>[9x]MDWHIAKHYDDILYYKAGGIAKIVINRPHKRNAFRPQTVFELYDAFCNAREDNRIGVVLLTGAGPHSDGKYAFCSGGDQSVRGEGGYIDDQGTPRLNVLDLQRLIRSMPKVVIALVAGYAIGGGHVLHLVCDLTIAADNAIFGQTGPKVGSFDGGFGSSYLARIVGQKKAREIWYLCRQYSAQEAERMGMVNTVVPVDRLEEEGIQWAKEILSKSPLAIRCLKAAFNADCDGQAGLQELAGNATLLYYMTEEGSEGKQAFLEKRPPDFSQYPWLP

1, 4-Dihydroxy-2-naphthoyl-CoA (DHNA-CoA) synthase, also called MenB, is responsible for conversion of o-succinylbenzoyl-CoA to DHNA-CoA in the biosynthesis of both vitamin K1 and K2. It catalyzes a multiple-step intramolecular Claisen condensation reaction involving two high energy oxyanion intermediates and two keto-enol tautomerizations in the formation of a naphthenoid ring. The first crystal structure of DHNA-CoA synthase from Mycobacterium tuberculosis shows that it forms two eclipsed trimers organized in a homologous hexameric assembly, in which each monomer is comprised of an N-terminal spiral core domain and a C-terminal helical domain conforming to a canonical crotonase fold. In addition to observing the folding of the active-site loop into a well-defined structure as previously seen in the substrate analog complex structure, we have identified a significant reorientation of the C-terminal helix as an additional conformational change caused by the small molecule ligands.

Through symmetry operation, all the trimers are found to be a part of the hexameric quaternary structure of scMenB. The active site of scMenB in complex with SA-CoA is also very similar to that of the ecMenB:HNA-CoA and scMenB:HNA-CoA complexes. However, no hydrogen-bonding network is found in the scMenB:SA-CoA structure. In addition, a bicarbonate ion is found in the place of the chloride ion in the ecMenB:HNA-CoA or scMenB:HNA-CoA structure. scMenB forms identical polar and nonpolar contacts with the adenylate moiety of HNA-CoA and SA-CoA in the complexes, but shows differences when compared to ecMenB. One of them is a strong hydrogen bond between the strictly conserved A-loop Arg-82 and the backbone carbonyl oxygen of the C-helix Gly-253, and the other polar loop-helix interaction is a hydrogen bond between the backbone carbonyl oxygen of Arg-82 and the side chain guanidinium group of Lys-257. For example, the side chain of scMenB Leu-261 on the C-helix forms hydrophobic contact with the A-loop, which replaces the interfacial hydrogen bond formed by the corresponding amino acid residue Asn-271 on the ecMenB C-helix. In addition, the adenylate 3′-phosphate group of the ligand is also stabilized by a ligand-induced salt bridge with the side chain of scMenB Lys-263, which is equivalent to ecMenB Lys-273. In the scMenB complexes, the lp−π interaction is formed between the purine moiety of the ligand and the backbone carbonyl oxygen of Lys-30 accompanying the hydrogen bond between the Lys-30 side chain and Ser-80.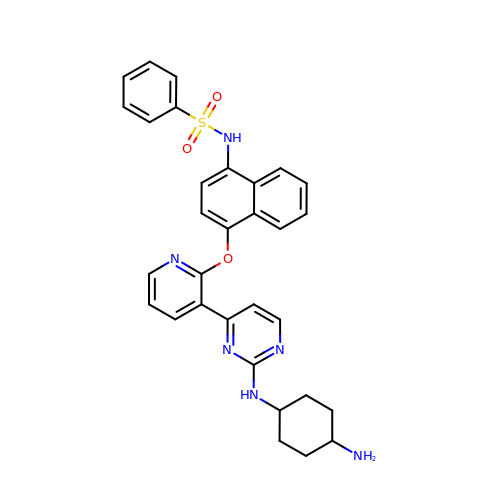N-{4-[(3-{2-[(trans-4-aminocyclohexyl)amino]pyrimidin-4-yl}pyridin-2-yl)oxy]naphthalen-1-yl}benzenesulfonamide | C31 H30 N6 O3 S | DXCOZKXVDMXKGR-HZCBDIJESA-N> MAQILPIRFQEHLQLQNLGINPANIGFSTLTMESDKFICIREKVGEQAQVVIIDMNDPSNPIRRPISADSAIMNPASKVIALKAGKTLQIFNIEM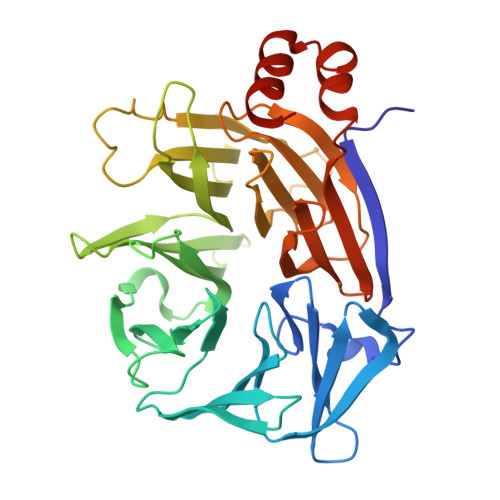KSKMKAHTMTDDVTFWKWISLNTVALVTDNAVYHWSMEGESQPVKMFDRHSSLAGCQIINYRTDAKQKWLLLTGISAQQNRVVGAMQLYSVDRKVSQPIEGHAASFAQFKMEGNAEESTLFCFAVRGQAGGKLHIIEVGTPPTGNQPFPKKAVDVFFPPEAQNDFPVAMQISEKHDVVFLITKYGYIHLYDLETGTCIYMNRISGETIFVTAPHEATAGIIGVNRKGQVLSVCVEEENIIPYITNVLQNPDLALRMAVRNNLAGAEELF> CHREPPPETPDINQLPPSILLKIFSNLSLDERCLSASLVCKYWRDLCLDFQFWKQLDLSSRQQVTDELLEKIASRSQNIIEINISDCRSMSDNGVCVLAFKCPGLLRYTAYRCKQLSDTSIIAVASHCPLLQK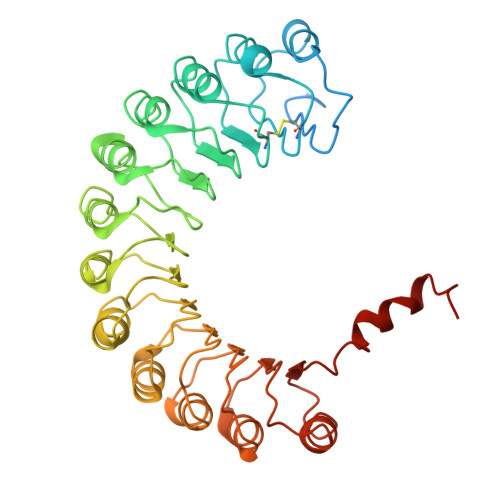VHVGNQDKLTDEGLKQLGSKCRELKDIHFGQCYKISDEGMIVIAKGCLKLQRIYMQENKLVTDQSVKAFAEHCPELQYVGFMGCSVTSKGVIHLTKLRNLSSLDLRHITELDNETVMEIVKRCKNLSSLNLCLNWIINDRCVEVIAKEGQNLKELYLVSCKITDYALIAIGRYSMTIETVDVGWCKEITDQGATLIAQSSKSLRYLGLMRCDKVNEVTVEQLVQQYPHITFSTVLQDCKRTLERAYQMGWTPNMSAASS> MEEDDNLKKGNERNKKKAIFSNDDFTGEDSLMEDHLELREKLSEDIDMIKTSLKNNLVCSTLNDNEILTLSNYMQFFVFKSGNLVIKQGEKGSYFFIINSGKFDVYVNDKKVKTMGKGSSFGEAALIHNTQRSATIIAETDGTLWGVQRSTFRATLKQLSNRNFNENRTFIDSVSVFDMLTEAQKNMITNACVIQNFKSGETIVKQGDYGDVLYILKEGKATVYINDEEIRVLEKGSYFGERALLYDEPRSATI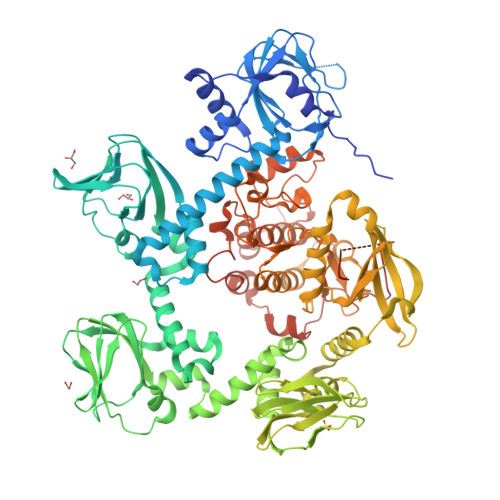IAKEPTACASICRKLLNIVLGNLQVVLFRNIMTEALQQSEIFKQFSGDQLNDLADTAIVRDYPANYNILHKDKVKSVKYIIVLEGKVELFLDDTSIGILSRGMSFGDQYVLNQKQPFKHTIKSLEVCKIALITETCLADCLGNNNIDASIDYNNKKSIIKKMYIFRYLTDKQCNLLIEAFRTTRYEEGDYIIQEGEVGSRFYIIKNGEVEIVKNKKRLRTLGKNDYFGERALLYDEPRTASVISKVNNVECWFVDKSVFLQIIQGPMLAHLEERIKMQDTKVEMDELETERIIGRGTFGTVKLVHHKPTKIRYALKCVSKRSIINLNQQNNIKLEREITAENDHPFIIRLVRTFKDSKYFYFLTELVTGGELYDAIRKLGLLSKSQAQFYLGSIILAIEYLHERNIVYRDLKPENILLDKQGYVKLIDFGCAKKVQGRAYTLVGTPHYMAPEVILGKGYGCTVDIWALGICLYEFICGPLPFGNDEEDQLEIFRDILTGQLTFPDYVTDTDSINLMKRLLCRLPQGRIGCSINGFKDIKDHPFFSNFNWDKLAGRLLDPPLVSKSETYAEDIDIKQIEEEDAEDDEEPLNDEDNWDIDF>[2x]MTDDSAVESKQKKSKIRKGHWIPVVA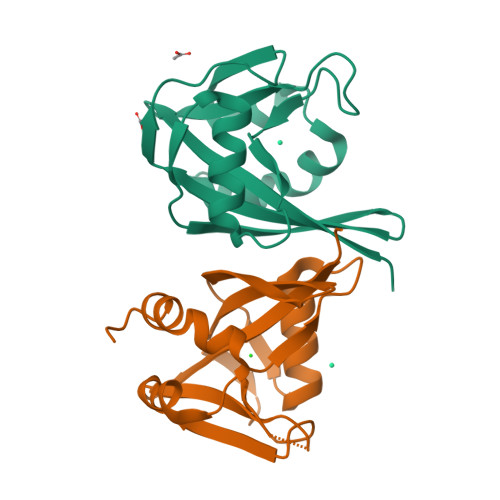GFLRKDGKILVGQRPENNSLAGQWEFPGGKIENGETPEEALARELNEELGIEAEVGELKLACTHSYGDVGILILFYEILYWKGEPRAKHHMMLEWIHPEELKHRNIPEANRKILHKIYKALGLEWRK6-~{tert}-butyl-8-fluoranyl-2-[3-(hydroxymethyl)-4-[1-methyl-6-oxidanylidene-5-(pyrimidin-4-ylamino)pyridin-3-yl]pyridin-2-yl]phthalazin-1-one | C28 H26 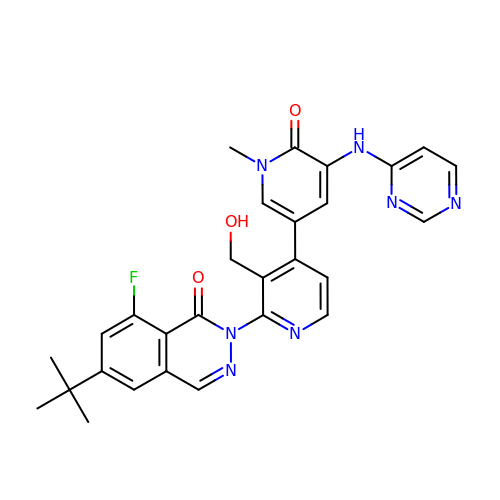F N7 O3 | QTEIEFCDHKXATA-UHFFFAOYSA-N Upon ligand binding, bone morphogenetic protein (BMP) receptors form active tetrameric complexes, comprised of two type I and two type II receptors, which then transmit signals to SMAD proteins. Here, using hydrogen deuterium exchange mass spectrometry (HDX-MS), small angle X-ray scattering (SAXS) and molecular dynamics (MD) simulations, combined with analysis of SMAD signaling, we show that the kinase domain of the type I receptor ALK2 and type II receptor BMPR2 form a heterodimeric complex via their C-terminal lobes. Formation of this dimer is essential for ligand-induced receptor signaling and is targeted by mutations in BMPR2 in patients with pulmonary arterial hypertension (PAH). We further show that the type I/type II kinase domain heterodimer serves as the scaffold for assembly of the active tetrameric receptor complexes to enable phosphorylation of the GS domain and activation of SMADs.

Remarkably, several of these mutations (C483R, D485G, D487V, A490D/V, and R491W/Q) cluster to the C1 dimer interface in the BMPR2 kinase domain, specifically at the αH-αI linker. Two sites of PAH mutations—D487 and D485—stand out because they make direct interactions with residues in ALK2 in the C1 dimer model. D485 was not included in our initial mutagenesis and was of particular interest. The D485G mutation is highly penetrant in PAH, and previous studies have shown its dominant-negative effect on BMPR2 signaling in complex with other type I receptors (ALK3 and ALK6) in cells. When the D485G mutation was introduced into BMPR2KD (BMPR2KD-D485G), the recombinant BMPR2KD-D485G did not dimerize with the wild-type ALK2KD. This mutation also had a dominant-negative effect on BMP4-dependent SMAD signaling by the ALK2/BMPR2KD-D485G full-length receptor complex. Due to prior speculations that loss of the acidic charge at residue 485 compromises the kinase fold, we obtained a crystal structure of the BMPR2KD-D485G kinase solved to 2.3 Å resolution. The BMPR2KD-D485G structure revealed an intact architecture of the kinase domain and overlaid with the recently reported structure of the wild-type BMPR2 kinase domain35 with an RMSD of 0.5 Å over 279 Cα atoms. Moreover, like other C-lobe mutants tested (BMPR2-EED and BMPR-EDE), the BMPR2KD-D485G mutant exhibited enzymatic activity comparable to the wild-type BMPR2KD. Thus, we conclude that the pathological effect of the D485G mutant of BMPR2 in PAH patients is due to loss of the receptor’s ability to engage in C-lobe-mediated heterodimers, which results in loss of downstream signaling.

>[2x]MGSSHHHHHHSSGENLYFQGHMMEAAASEPSLDLDNLKLLELIGRGRYGAVYKGSLDERPVAVKVFSFANRQNFINEKNIYRVPLMEHDNIARFIVGDERVTADGRMEYLLVMEYYPNGSLCKYLSLHTSDWVSSCRLAHSVTRGLAYLHTELPRGDHYKPAISHRDLNSRNVLVKNDGTCVISDFGLSMRLTGNRLVRPGEEDNAAISEVGTIRYMAPEVLEGAVNLRDCESALKQVDMYALGLIYWEIFMRCTDLFPGESVPEYQMAFQTEVGNHPTFEDMQVLVSREKQRPKFPEAWKENSLAVRSLKETIEDCWGQDAEARLTAQCAEERMAELMMIWERNKSVSPTVNPMSTAMQNER> AFQAKLDT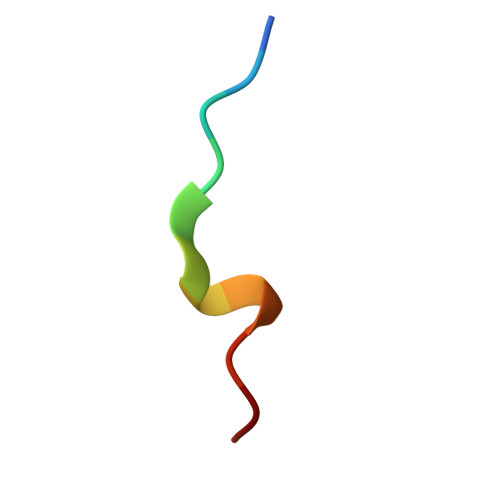FLWS NICOTINAMIDE ADENINE DINUCLEOTIDE ACETONE 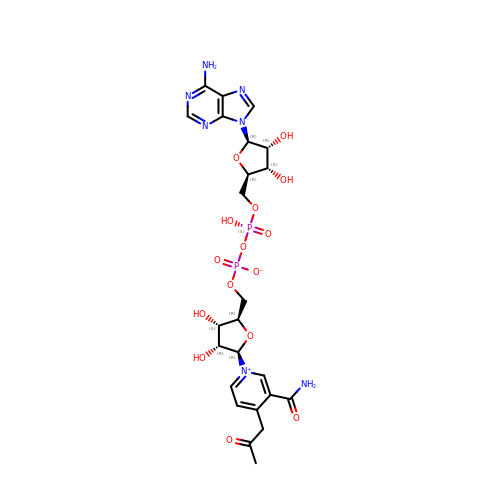ADDUCT | C24 H31 N7 O15 P2 | SGHBFOOIAAJJMI-YDKVLQLQSA-N> GAMAVLDPEVAQLLSQANEAFVRNDLQVAERLFNEVIKKDARNFAAYETLGDIYQLQGRLNDCCNSWFLAAHLNASDWEFWKIVAILSADLDHVRQAIYCFSRVISLNPMEWESIYRRSMLYKKTGQLARALDGFQRLYMYNPYDANILRELAILYVDYDRIEDSIELYMKVFNANVERREAILAALENALDSSDEESAAEGEDADEKEPLEQDEDRQMFPDINWKKIDAKYKCIPFDWSSLNILAELFLKLAVSEVDGIKTIKKCARWIQRRESQTFWDHVPDDSEFDNRRFKNSTFDSLLAAEKEKSYNIPIDIRVRLGLLRLNTDNLVEALNHFQCLYDETFSDVADLYFEAATALTRAEKYKEAIDFFTPLLSLEEWRTTDVFKPLARCYKEIESYETAKEFYELAIKSEPDDLDIRVSLAEVYYRLNDPETFKHMLVDVVEMR

Recruitment of Pol III to these genes requires the essential transcription factors TFIIIB and TFIIIC2. The six subunits of yeast TFIIIC are partitioned into two DNA-binding subcomplexes (τA and τB). The binding of these intragenic promoters by TFIIIC permits the assembly of TFIIIB, upstream of the transcription start site, which subsequently leads to the recruitment of Pol III, the formation of a PIC and finally to transcription. A genetic study suggests that the two largest TFIIIC subunits, τ138 and τ131, are responsible for connecting τA and τB16.

Given that our crosslinking data implicated the TPR array of τ131 in connecting τA and τB, and the reported importance of this region for TFIIIB assembly, we determined the crystal structure of the TPR array (residues 123–566) in two different space groups (P62 and P43). We were able to collect diffraction data up to 3.15 Å (P62) and 3.4 Å (P43) resolution. The lower-resolution structure was solved by multiple isomorphous replacement with anomalous signal (MIRAS), using anomalous signal from crystals prepared with selenomethionine substituted proteins or native crystals soaked with p-chloromercuribenzensulfonic acid to final Rwork/Rfree values of 20.9%/24.5% The higher-resolution structure was solved using selenomethionine substituted protein in single anomalous dispersion (SAD) experiments and subsequently refined to Rwork/Rfree values of 25.0%/28.7%. The structure reveals the presence of 10 TPR repeats, while only nine TPR repeats had been predicted. Rather than forming an extended super-helix, the TPR array is instead separated into two ‘arms' by a central region that contains an extended helix and a disordered coil we call ‘ring' domain. This insertion causes a bend in the TPR array, positioning the TPRs of the right arm closer to the TPRs of the left arm. A superimposition of the two crystal forms and an analysis of temperature factors reveal flexibility at TPRs 1–3, 8–10 and residues at the extremes of the extended helix. Surface analysis of the TPR array shows that the inner groove is lined with patches of conserved, often acidic surface residues that may bind to the predicted basic surface residues of τ138. To our knowledge, this is the first time that a loss of interaction by both of these mutations has been probed directly using purified proteins. These results suggest that the binding hotspot for τ138 thus overlaps with that of a binding site for Bdp1.>MKFTLLSVVAIAAAASDSYAAPAASSLAGPVTTGVFSAVSAIPSFATNLSGQVASATSTVLSGSTASGSSATAAPSASASGASSMQSMASSLSGSAFSPSSMMPIASGNMTMPNMTSSASASSAASTATGVAGGAGSNSSSSCAPTSLPASATELPTTVPTGTVITGDYTGSYRPQVHYSPPKGFMNDPNGCHRDRNGTYHLYYQYNPLEYVAGNQHWGHATSDDLYHWTNQPIAIFPPNSTSQVFSGSAVLDPNNTSGFFPNTTDGVVAVYTLNTPTLQVQEVAYSTDGGYNFTPYENNPVLSVGSNQFRDPKVFWYEDHWVMAVAAANDFTIEIYTSPNLTSWTFASNFTHHGLLGLAYECPNLVQVPFQDDPSKSAWLMYISINPGAPLGGSVGQYFPGDFNGTHFVAYDSAARIADFAKDNYASQWFADTENGESISIAWASNWQYTQQVPTSAQAFRSAMSLPRRNYLTNITRLGWDLVSLPYDLSPVVGPSLLSSSEANSTADVDF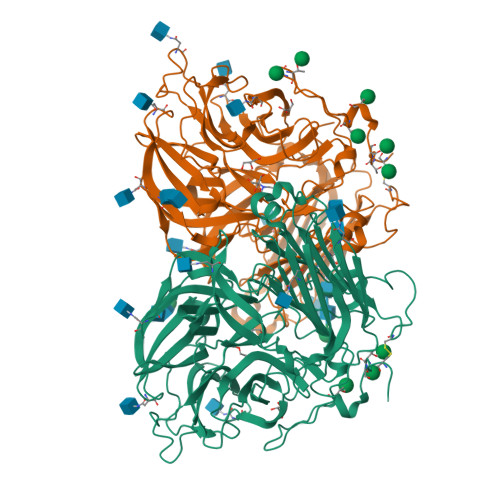TNVTSNAVWFSLNVTLPDAAIQNASLISADASINITFLPSTKCSSSSGSGSDSPAATLTYFYAGLTNGALALTRPAASSSWGAENPFFTDKFSYTLVDPLTSLVGVFDRSMLEVFVNEGAHSATMLVFPDSPVGSMKVATGGLPEGTQVNLQVNGLESTWQSS[2x]>[6x]NVEEETKYIELMIVNDHLMFKKHRLSVVHTNTYAKSVVNMADLIYKDQLKTRIVLVAMETWATDNKFAISENPLITLREFMKYRRDFIKEKSDAVHLFSGSQFESSRSGAAYIGGICSLLKGGGVNEFGKTDLMAVTLAQSLAHNIGIISDKRKLASGECKCEDTWSGCIMGDTGYYLPKKFTQCNIEEYHDFLNSGGGACLFNKPSKLLDPPECGNGFIETGEECDCGTPAECVLEGAECCKKCTLTQDSQCSDGLCCKKCKFQPMGTVCREAVNDCDIRETCSGNSSQCAPNIHKMDGYSCDGVQGICFGGRCKTRDRQCKYIWGQKVTASDKYCYEKLNIEGTEKGNCGKDKDTWIQCNKRDVLCGYLLCTNIGNIPRLGELDGEITSTLVVQQGRTLNCSGGHVKLEEDVDLGYVEDGTPCGPQMMCLEHRCLPVASFNFSTCLSSKEGTICSGNGVCSNELKCVCN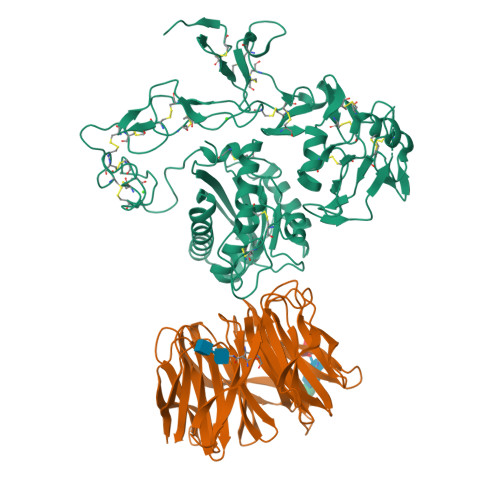RHWIGSDCNTYFPHNDDAKTGITLSGKHHHHHH;>[6x]DAAQPATEFAKSQDLPYQSLSIDTFSYLNDEYVVIAQPFTGKCIFLEWDHVEKTFRNYDNITGTSTVVCKPIVIETQLYVIVAQLFGGSHIYKRDSFANKFIKIQDIEILKIRKPNDIETFKIENNWYFVVADSSKAGFTTIYKWNGNGFYSHQSLHAWYRDTDVEYLEIVRTPQTLRTPHLILSSSSQRPVIYQWNKATQLFTNQTDIPNMEDVYAVKHFSVKGDVYICLTRFIGDSKVMKWGGSSFQDIQRMPSRGSMVFQPLQINNYQYAILGSDYSFTQVYNWDAEKAKFVKFQELNVQAPRSFTHVSINKRNFLFASSFKGNTQIYKHVIVDLSAKHHHHHH>MAPFPEEVDVFTAPHWRMKQLVGLYCDKLSKTNFSNNNDFRALLQSLYATFKEFKMHEQIENEYI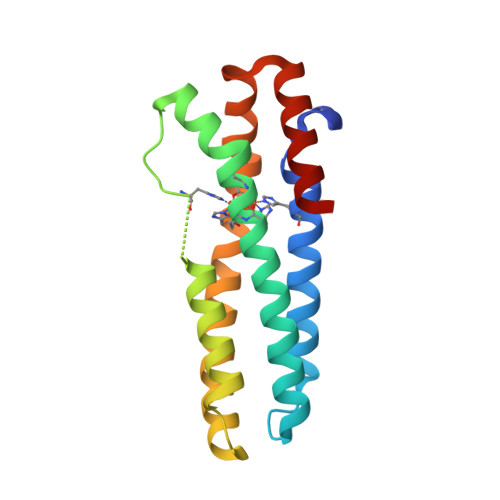IGLLQQRSQTIYNVHSDNKLSEMLSLFEKGLKNVKNEYEQLNYAKQLKERLEAFTRDFLPHMKEEEEVFQPMLMEYFTYEELKDIKKKVIAQHCSQ[2x]> TQKPSLYRVLILNDDYTPMEFVVYVLERFFNK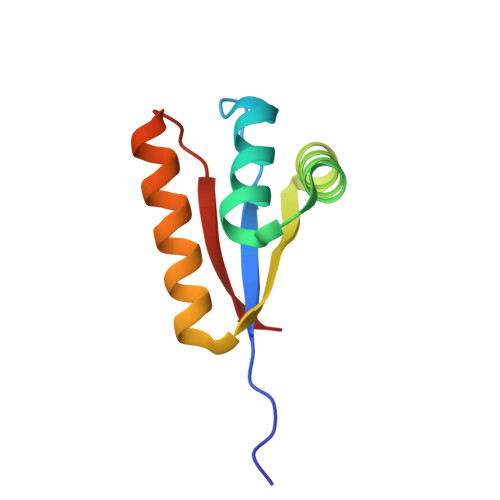SREDATRIMLHVHQNGVGVCGVYTYEVAETKVAQVIDSARRHQHPLQCTMEKD> PIFLNVLEAIEPGVVCAGHDNNQPDSFAALLSSLNELGERQLVHVVKWAKALPGFRNLHVDDQMAVIQYSWMGLMVFAMGWRSFTNVNSRMLYFAPDLVFNEYRMHKSRMYSQCVRMRHLSQEFGWLQITPQEFLCMKALLLF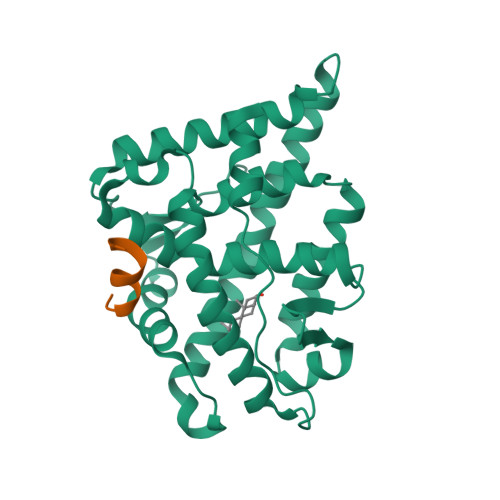SIIPVDGLKNQKFFDELRMNYIKELDRIIACKRKNPTSCSRRFYQLTKLLDSVQPIARELHQFTFDLLIKSHMVSVDFPEMMAEIISVQVPKILSGKVKPIYFHT;> PSILKKILLE> GETKVIYHLDEEETP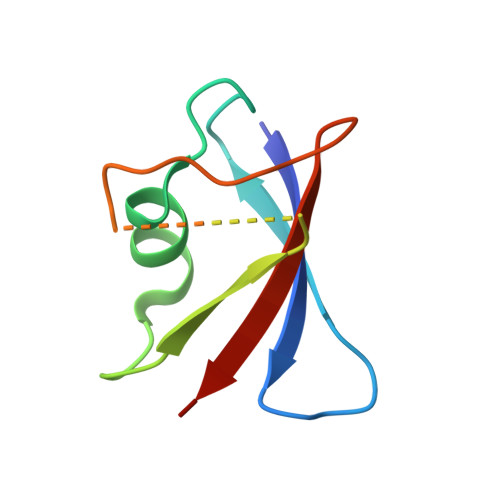YLVKIPVPAERITLGDFKSVLQRPAGAKYFFKSMDQDFGVAAEEISDDNARLPCFNGRVVSWLVSSD> GAMPDG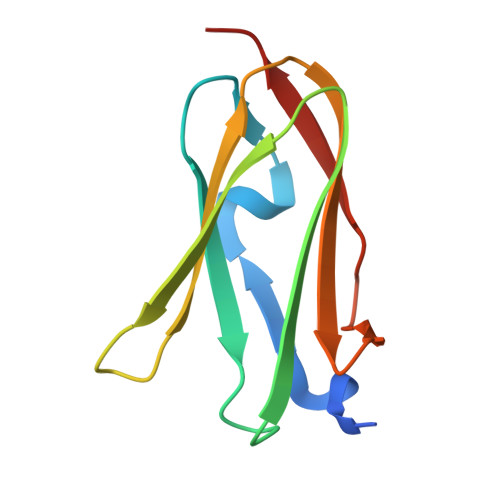GAHKVRAGGPGLERAEAGVPAEFSIWTREAGAGGLAIAVEGPSKAEISFEDRKDGSCGVAYVVQEPGDYEVSVKFNEEHIPDSPFVVPVASPS> MSNYVIQADQQLLDALRAHYEGALSDRLPAGALFAVKRPDVVITAYRSGKVLFQGKAAEQEAAKWISGASASNETADHQPSALAAHQLGSLSAIGSDEVGTGDYFGPIVVAAAYVDRPHIAKIAALGVKDSKQLNDEAIKRIAPAIMETVPHAVTVLDNPQYNRWQRSGMPQTKMKALLHNRTLVKLVDAIAPAEPEAIIIDEFLKRDSYFRYLSDEDRIIRERVHCLPKAESVHV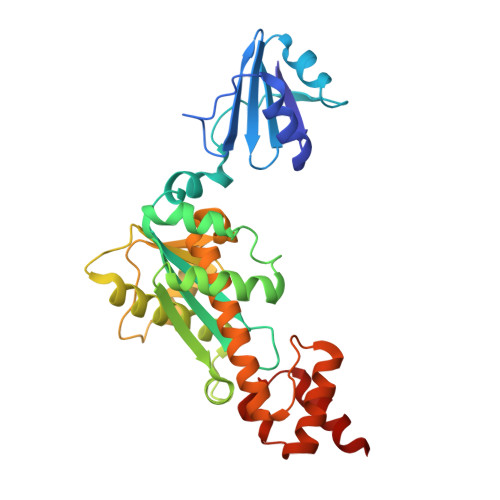SVAAASIIARYVFLEEMEQLSRAVGLLLPKGAGAIVDEAAARIIRARGEEMLETCAKLHFANTKKALAIAKRRK> TTNPVDLWSAPSSQARLEKEYFDQHFGPFFRTEQLIIRAPLTDKHIYQPYPSGADVPFGPPLDIQILHQVLDLQIAIENITASYDNETVTLQDICLAPLSPYNTNCTILSVLNYFQNSHSVLDHKKGDDFFVYADYHTHFLYCVRAPASLNDTSLLHDPCLGTFGGPVFPWLVLGGYDDQNYNNATALVITFPVNNYYNDTEKLQRAQAWEKEFINFVKNYKNPN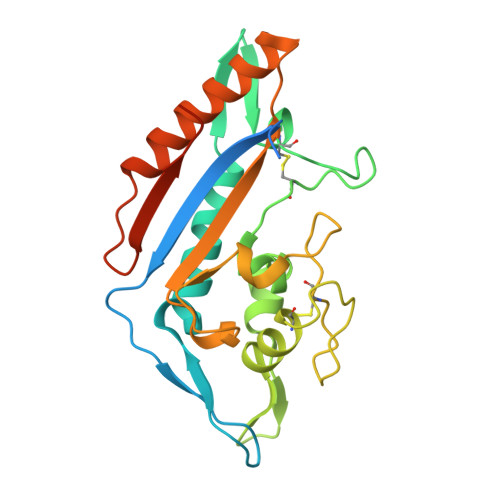LTISFTAERSIEDELNRESDSD>SMPRVDFPRSRLRFKEKLGEGQFGEVHLCEVDSPQDLVSLDFPLNVRKGHPLLVAVKILRPDATKNARNDFLKEVKIMSRLKDPNIIRLLGVCVQDDPLCMITDYMENGDLNQFLSAHQLEDKAAEGAPGDGQAAQGPTISYPMLLHVAAQIASGMRYLATLNFVHRDLATRNCLVGENFTI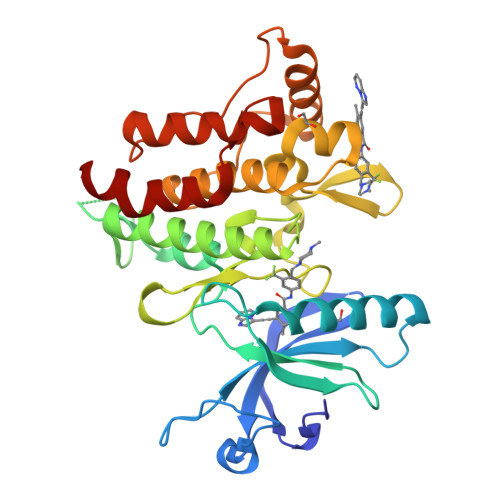KIADFGMSRNLYAGDYYRVQGRAVLPIRWMAWECILMGKFTTASDVWAFGVTLWEVLMLCRAQPFGQLTDEQVIENAGEFFRDQGRQVYLSRPPACPQGLYELMLRCWSRESEQRPPFSQLHRFLAEDALNTV[2x]2-[4-(phenylmethyl)piperidin-1-yl]ethanamine 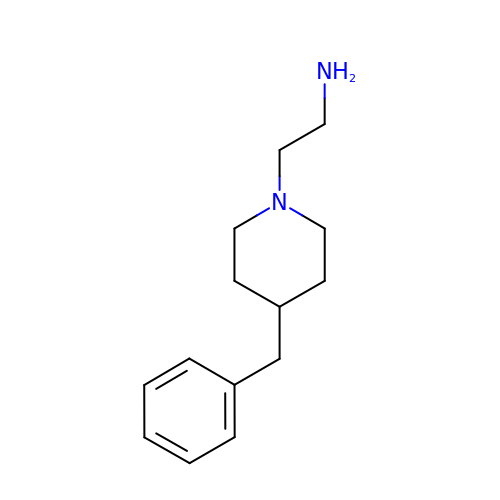| C14 H22 N2 | PCNDXYHWLSHXMV-UHFFFAOYSA-N>KLNMLKPDSDLCLKFAMLCTLNDKCDRLRKAYGEACSGPHCQRHVCLRQLLTFFEKAAEPHAQGLLLCPCAPNDRGCGERRRNTIAPNCALPPVAPNCLELRRLCFSDPLCRSRLVDFQTHCHPMDILGTCATEQSRCLRAYLGLIGTAMTPNFVSNVNTSVALSCTCRGSGNLQEECEMLEGFFSHNPCLTEAIAAKMRFHSQLFSQDWPHP[2x];>[2x]DPGCRLRSQLVPVRALGLGHRSDELVRFRFCSGSCRRARSPHDLSLASLLGAGALRPP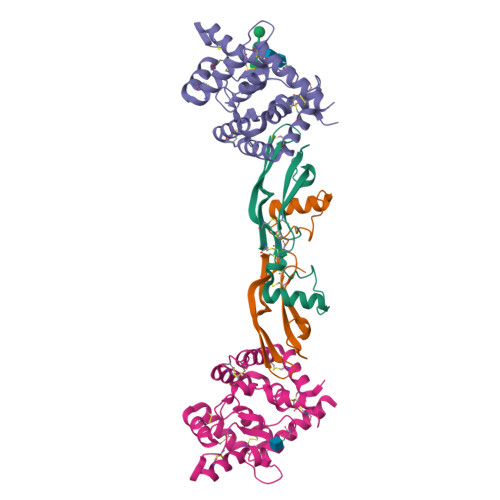PGSRPVSQPCCRPTRYEAVSFMDVNSTWRTVDRLSATACGCLG> SCFALISGTANQVKCYRFRVKKNHRHRYENCTTTWFTVADNGA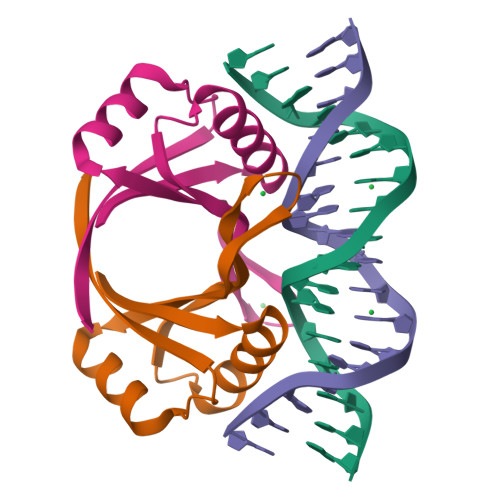ERQGQAQILITFGSPSQRQDFLKHVPLPPGMNISGFTASLDF>MTSAEMTSPNNNSEHQAIAKMRTMIEGFDDISHGGLPIGRSTLVSGTSGTGKTLFSIQFLYNGIIEFDEPGVFVTFEETPQDIIKNARSFGWDLAKLVDEGKLFILDASPDPEGQEVVGGFDLSALIERINYAIQKYRARRVSIDSVTSVFQQYDASSVVRRELFRLVARLKQIGATTVMTTERIEEYGPIARYGVEEF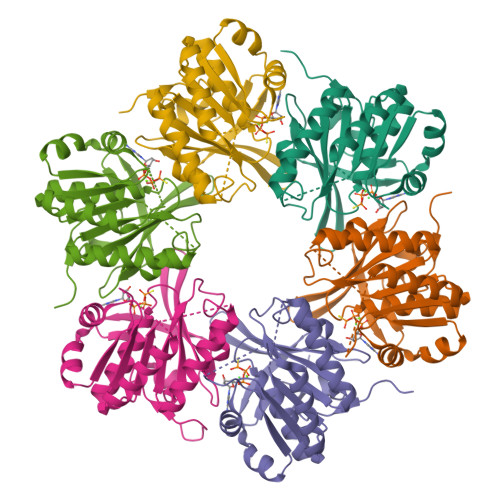VSDNVVILRNVLEGERRRRTLEILKLRGTSHMKGEYPFTITDHGINIFPLGAMR[6x]> TEVTDCKGDAESSLTTALSNAAKLANQAAEAAESGDESKFEEYFKTTDQQTR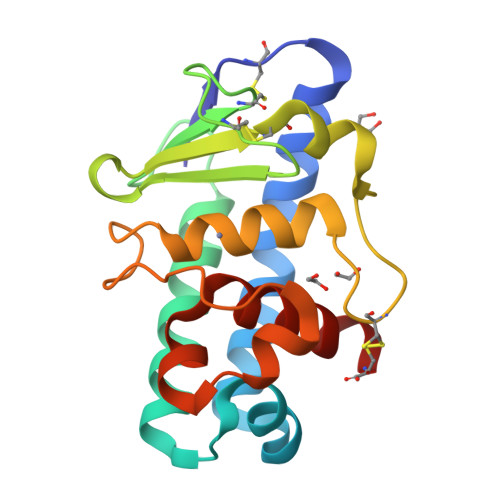TTVAERLRAVAKEAGSTSGGSTTYHCNDPYGYCEPNVLAYTLPSKNEIANCDIYYSELPPLAQKCHAQDQATTTLHEFTHAPGVYQPGTEDLGYGYDAATQLSAQDALNNADSYALYANAIELKC>[2x]EFSPAAAPPTLPPYFMKGSIIQLANGELKKVEDLKTEDFIQSAE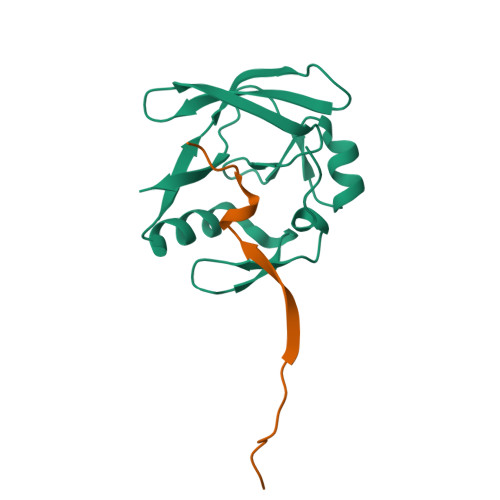ISNDLKIDSSTVERIEDSHSPGVAVIQFAVGEHRAQVSVEVLVEYPFFVFGQGWSSCCPERTSQLFDLPCSKLSVGDVCISLTLK;>MFVWTNVEPRSVAVFPWHSLVPFLAPSQ[2x]>MELFDENYYAKAVANIIGEVKDPIMYKWFSPDQIEDVDLQMGYQKTVKWDAFLNANPTTIANEVNTISTIGFSSEVVRLNYLKLQYKFRHLKQTSEKFYTSDSYIGDINNNLLPFAQAYKLASSEIIKLINHFVLTGTVSIQKDGKNQKRLLPNMYGLLNMPEQIKEEVASGDKDKMDKIFEKI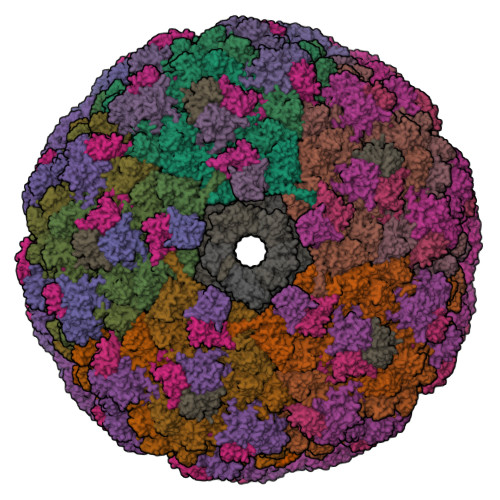EAGLSKLELGDEFSTPMMVIVDPATSLKLVKPYAAAQGAASSCEKWEDVLIQTIKAINNREDVYIETSNLLKHKILIYPLNSELIKFKPSKYMLPTPNEQVDKDSTDVAHSYIDFVLGGLLATRKTILQVNIKQS[130x];>MSDITKIKQEFDKKVAEIQALMKNPQQDSGLLSNSIDFRDQNLIFSNSGGVCTSSKDKIENYPAKGYPYKRGVKLSFGDGTTELEVEAGGGDDLYGVCSDIDEFSGMATVIPITNNFTGYLTLKKDGQNGVNPGDKLNFNQHGELEKVTGAQKSVNAIALSKAHKLTEDLFIVLASVFGNRAIKG[75x];>[35x]MGDTTQLVKEYQEKRSKLEKFMKNPQHDASLLSNSNEFRDKNVEFFASGGTRTSKFDKLENHPFLGYPYKRGVKRVIQEAQDNQSHYEPHVEAGGGEDLYGICIDIDEFSKTATIVPITNNFEGYLVAKDSTVKVKDKLIFNKDGALEKVTGAPNKATINATALTDAKQISNEVYLVKVAVFGNKAMSRN;>MTEKEEKEDLQAQDKEEQQIKADTKVISVQEFEEYMRFKEQANSKSKETSRDLSINERITKELAEVEERERIEKQLLLEAERINEIDTLAKAHLSNHFNKEVLLAKGYTLKDIMQAQRRELVRKFVPIEQIKAIAKVSDISHIDGEILEQLVSLAKVNIKLRKNASSSSSSVDSIKGNIAIKSEERASLLDSNFVPINFTEFVQAISNTYKQRRIQFYENLKRHKRTSIA[253x];>[5x]MALKGNMQVENLEAVEDPQVDLGAQVSAAPRAKRQARQAEDVQGEDPYLESISELDDVLLKFKKYSKSMSSIENKVFSSSSGCFKSKNERVDAYSFACSSYTDKIEEYLYDPANSFPYKRGVKLVPKENSIYVEVGADTDMYGICVDVCEFSCTAYVLPITNNFEGYLVTRNPSIKIGEILDINNNGVIIKAGGGPPTAINIYALSDSFTINFAPEDGNQDQNRYPRQEYSINLIKVAIFGNRGLEKTVNPDGG;>[12x]MCDLRKTKLIDKISSLELYKYSIFFRNYIENVAEDCLKNGLILESAAHNVSEVELARLKVQLKNALLNCIISYRFHGIGYVLVKTKDTLIDLEQPVNIELPIGFEYLDYEYVRDLGVDFDHITYKVKSNNKNNSLDAVKIHKSRLIIYENFDYILKRYVPCYTESFLLDIYLFEKIYVEIERRIENHNFLFYKDESLVQLQDALSSATTSLSALTQSNNDRGSGILSSFLRKQNSNNHSKDISNLRNLNDSLSQELARLKSNLNNEGMFYTATPSASLEVIKYDLSYLKEALALIKAKIGADTKEPLTRSFNEQAKGLGNDGKGDRSNYYDFLKGVQEQVENSCNLKLTKYFGLDMKFNSLIMLSEEQKVERDIKLIELYSKYNQLIQSSSFNNEELAMLKEKLFSF> MKFGLFFLNFMNSKRSSDQVIEEMLDTAHYVDQLKFDTLAVYENHFSNNGVVGAPLTVAGFLLGMTKNAKVASLNHVITTHHPVRVAEEACLLDQMSEGRFAFGFSDCEKSADMRFFNRPTDSQFQLFSECHKIINDAFTTGYCHPNNDFYSFPKISVNPHA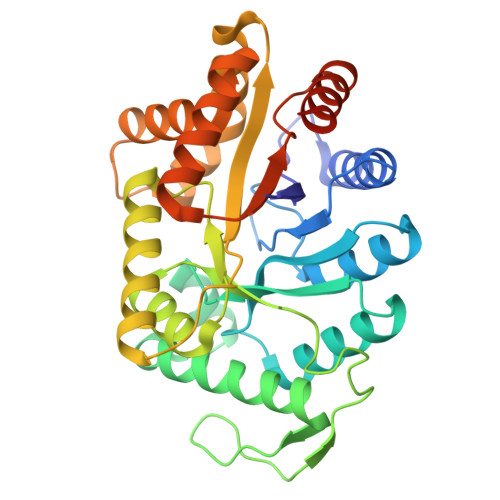FTEGGPAQFVNATSKEVVEWAAKLGLPLVFRWDDSNAQRKEYAGLYHEVAQAHGVDVSQVRHKLTLLVNQNVDGEAARAEARVYLEEFVRESYSNTDFEQKMGELLSENAIGTYEESTQAARVAIECCGAADLLMSFESMEDKAQQRAVIDVVNANIVKYHSLEHHHHHH>[3x]GHMKGLTEKLMI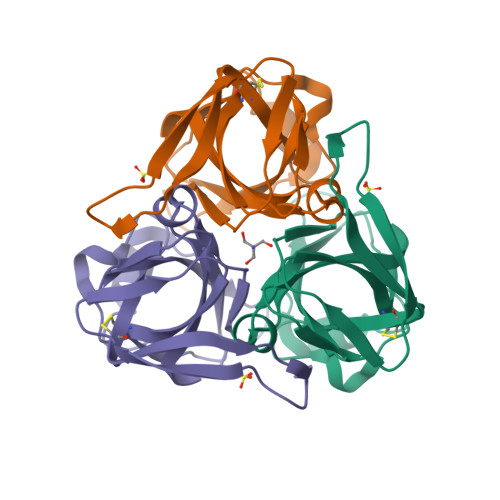LSHQSIKNLLGKVILNYSEENVRENGYDLRICGDKYYELVQGAELPEKKATLREIEFKERAILSANHTYLFESCEEFNMPADLAVLITLKSTLARNGFLAPPTVIDAGYKGKVNVAITAVYNSSLKKGMATHHLIFLKLDKPTERLYNGKYQGGILI2-cyclopentyl-4-(5-phenylfuro[2,3-b]pyridin-3-yl)benzoic acid | C25 H21 N O3 | 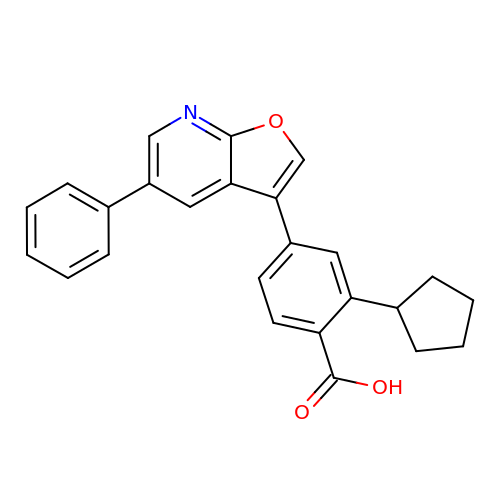GZZXEPJJXLJJEJ-UHFFFAOYSA-N>MGKYFGTDGVRGVANSELTPELAFKVGRFGGYVLTKDKQRPKVLIGRDTRISGHMLEGALVAGLLSIGAEVMRLGVISTPGVSYLTKAMDAEAGVMISASHNPVQDNGIKFFGGDGFKLSDEQEAEIERLMDEPEDKLPRPVGADLGLVNDYFEGGQKYLQFLKQTADEDFTGIHVALDCANGATSSLATHLFADLDADVSTMGTSPNGLNINDGVGSTHPEALSAFVKEKNADLGLAFDGDGDRLIAVDEKGNIVDGDQIMYICSKHLKSEGRLKDDTVVSTVMSNLGFYKALEKEGIKSVQTAVGDRYVVEAMKKDGYNVGGEQSGHLIFLDYNTTGDGLLSAIMLMNTLKATGKPLSELAAEMQKFPQLLVNVRVTDKYKVEENEKVKAVISEVEKEMNGDGRILVRPSGTEPLVRVMAEAKTKELCDEYVNRIVEVVRSEMGLELVPRGSSGLEHHHHHH[6x];>EAQQKTIEAITKAINYMAKRRIGALLTIERDTGMGDYIETGIPLNAKVSSELLINIFIPNTPLHDGAVIMKNNEIAAAACYLPLSESPFISKELGTRHRAAVGISEVTDSLTIIVSEETGGVSVAKNGDLHRELTEEALKEMLEAEFKK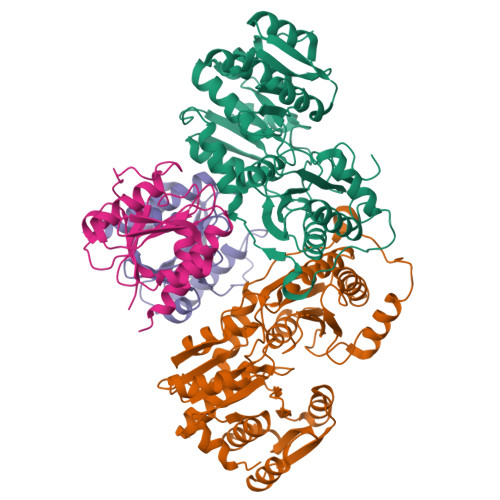NTRDTSSNRWYWRGKKNG[6x]>[8x]MPPETATNPKDARHDGWQTLKRFLPYLWPADNAVLRRRVVGAILMVLLGKATTLALPFAYKKAVDAMTLGGGAQPALTVALAFVLAYALGRFSGVLFDNLRNIVFERVGQDATRHLAENVFARLHKLSLRFHLARRTGEVTKVIERGTKSIDTMLYFLLFNIAPT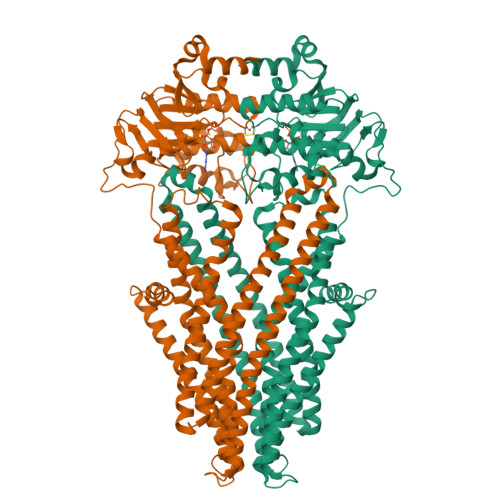VIELTAVIVIFWLNFGLGLVTATILAVIAYVWTTRTITEWRTHLREKMNRLDGQALARAVDSLLNYETVKYFGAESREEARYASAARAYADAAVKSENSLGLLNIAQALIVNLLMAGAMAWTVYGWSQGKLTVGDLVFVNTYLTQLFRPLDMLGMVYRTIRQGLIDMAEMFRLIDTHIEVADVPNAPALVVNRPSVTFDNVVFGYDRDREILHGLSFEVAAGSRVAIVGPSGAGKSTIARLLFRFYDPWEGRILIDGQDIAHVTQTSLRAALGIVPQDSVLFNDTIGYNIAYGRDGASRAEVDAAAKGAAIADFIARLPQGYDTEVGERGLKLSGGEKQRVAIARTLVKNPPILLFDEATSCLDTRTEQDILSTMRAVASHRTTISIAHRLSTIADSDTILVLDQGRLAEQGSHLDLLRRDGLYAEMWARQAAESAEVSEAAEHHHHHH>MNLDVWQHIRQEAKELAENEPMLASFFHSTILKHQNLGGALSYLLANKLANPIMPAISLREIIEEAYQSNPSIIDCAACDIQAVRHRDPAVELWSTPLLYLKGFHAIQSYRITHYLWNQNRKSLALYLQNQISVAFDVDIHPAAKIGHGIMFDHATGIVVGETSVIENDVSILQGVTLGGTGKESGDRHPKVREGVMIGAGAKILGNIEVGKYAKIGANSVVLNPVPEYATAAGVPARIVSQDKAAK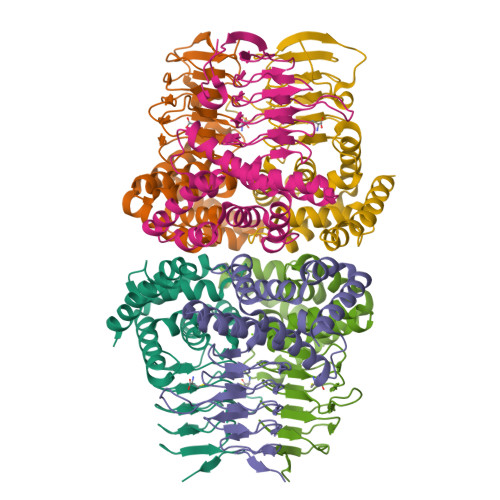PAFDMNQYFIGIDDGMNLNI[2x]>SMGFWEASSRGGGAFSGGEDASEGGAEEGAGGAGGSAGAGEGPVITALTPMTIPDVFPHLPLIAITRNPVFPRFIKIIEVKNKKLVELLRRKVRLAQPYVGVFLKRDDSNESDVVESLDEIYHTGTFAQIHEMQDLGDKLRMIVMGHRRVHISRQLEVEPEEPEAENKHKPRRKSKRGKKEAEDELSARHPAELAMEPTPELPAEVLMVEVENVVHEDFQVTEEVKALTAEIVKTIRDIIALNPLYRESVLQMMQAGQRVVDNPIYLSDMGAALTGAESHELQDVLEETNIPKRLYKALSLLKKEFELSKLQQRLGREVEEKIKQTHRKYLLQEQLKIIKKELGLEKDDKDAIEEKFRERLKELVVPKHVMDVVDEELSKLGLLDNHSSEFNVTRNYLDWLTSIPWGKYSNENLDLARAQAVLEEDHYGMEDVKKRILEFIAVSQLRGSTQGKILCFYGPPGVGKTSIARSIARALNREYFRFSVGGMTDVAEIKGHRRTYVGAMPGKIIQCLKKTKTENPLILIDEVDKIGRGYQGDPSSALLELLDPEQNANFLDHYLDVPVDLSKVLFICTANVTDTIPEPLRDRMEMINVSGYVAQEKLAIAERYLVPQARALCGLDESKAKLSSDVLTLLIKQYCRESGVRNLQKQVEKVLRKSAYKIVSGEAESVEVTPENLQDFVGKPVFTVERMYDVTPPGVVMGLAWTAMGGSTLFVETSL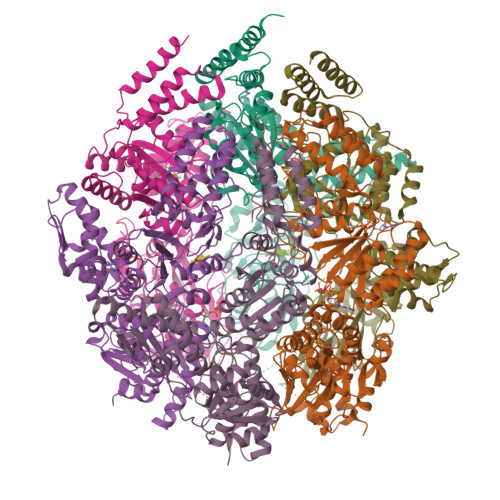RRPQDKDAKGDKDGSLEVTGQLGEVMKESARIAYTFARAFLMQHAPANDYLVTSHIHLHVPEGATPKDGPSAGCTIVTALLSLAMGRPVRQNLAMTGEVSLTGKILPVGGIKEATIAAKRAGVTCIVLPAENKKDFYDLAAFITEGLEVHFVEHYREIFDIAFPDEQAEALAVER[6x]>ADTKAKLTLDGDTAVELDVLKGTLGQDVIDIRTLGSKGVFTFDPGFTSTTSCESKITFIDGDEGILLHRGFPIDQLATDSNYLEVCYILLNGEKPTQEQYDEFKTTVTRHTMIHEQITRLFHAFRRDSHPMAVMCGITGALAAFYHDSLDVNNPRHREIAAFRLLSKMPTMAAMCYKYSIGQPFVYPRNDLSYAGNFLNMMFSTPCEPYEVNPILERAMDRILILHADHEQNASTSTVRTAGSSGANPFACIAAG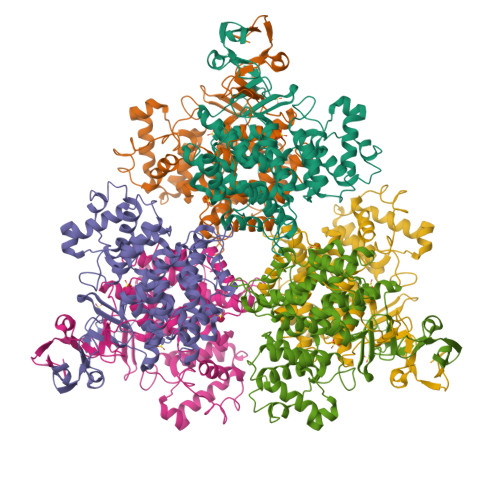IASLWGPAHGGANEAALKMLEEIGKKENIPEFVRRAKDKNDSFRLMGFGHRVYKNYDPRATVMRETCHEVLKELGTKDDLLEVAMELENIALNDPYFIEKKLYPNVDFYSGIILKAMGIPSSMFTVIFAMARTVGWIAHWSEMHSDGMKIARPRQLYTGYEKRDFKSDIKR[2x]>TEGRVQHFTGYIEDGRGIFYSLPDMKQGDIIYASMQNTGGNLDPLVGIM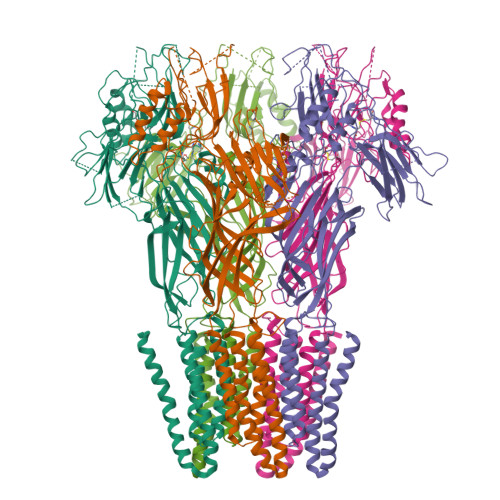AEEIDPAVSLGQVLEKALASENDLISELTAVADRIFLGWDDDGGKGYSASLEFTIPRDGTYHIFAGSTITNQRLDKFQPTYTTGSFQLILGLNAPQVISGEGEPEGEVFASLASLEIKPEAHVQELEIRLDKDTRYLTQHTRNLQPGDTFHALVEPIGEAPLPRLRLTDSGGKPLAFGLIDQPGESVELNYTCDQDICELVVHVDGTDGQKDSGEAVYRLLVGINAPNLRESGQTPVGSSVFLESDLVTVGLAVDQIVGVDQRSENFSVVGTLKLSWHDPKLGFSPDQCGCTVKSFEDASIRAVAGEINLPLPSFSFYNQQGNRWSQNQVIFVTPDGRASYFERFTVTLQAPDFDFLAYPFDRQKFSIKVDLAVPTNMFIFNEIERFQQVVGDQLGEEEWVVTSYSQEITEVPFERGSTNSRFTTTLLVKRNLEYYILRIFVPLFLIISVSWVIFFLKDYGRQLEVASGNLLVFVAFNFTISGDLPRLGYLTVLDRFMIVSFCLTAIVVLISVCQKRLGAVGKQAVAAQIDTWVLVIYPLVYSLYIIWVYLRFFTDHIGW[5x]>[2x]GAMSE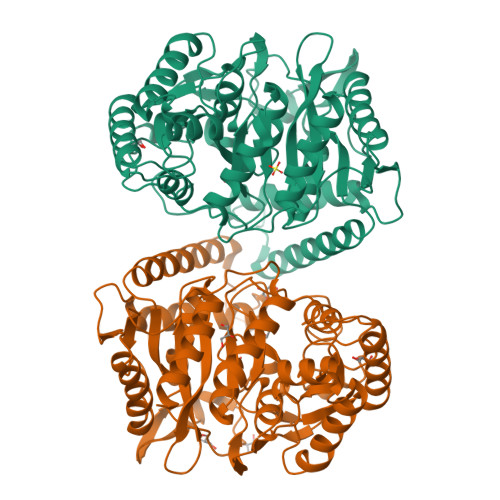LSAIETAAAIAGGSMTALEACDAAIARIEQRDGPINAVVVRDFDRARDAAKAADAEIAAAVRKPLLGVPMTIKESFDIAGLPTSWGFAEHADHIATADSLVVSRLKAAGAVFLGKSNIPVGLADWQSVNPNYGRTNNPHDHSRSAGGSSGGAAAALAAGMVPLEYGSDIGGSIRVPAHFCGVWGLKTTFDAVSLEGHYFPRTDSAKADLSVVGPMARTPADLALALDITSKVPLPQSRIANLSGLRILLLTAHPETVADSATISAVERAAAACEASGATVATSSPDLPDLSALVADYTRMLLVVLARGLAPEGTEPVSLNAWYAMLDDQARMMRAFDRLFESFDAIFCPVLGTTAFAHSDEPDWAKRSLSIDGGIAPFAAQLGWISMATYGGMPALSMPLGADGNGLPINLQIITRNWSDHDAIRIGALVAEALDR>MGSSHHHHHHGSGENLYFQSNQPLKIVVPFSAGGTADVLPRLVAEKIRADYAGGVIIENKPGAGGNIGADLVFRAPPDGMTVLASPPGPIAINHNLYQKLSFDPTRWVPVTILATVPNVLVINPKLPVKSLGEFIAYAKANPKKVTVATQGDGSTSHLTAAMFMQLTGTELTVIPYKGTA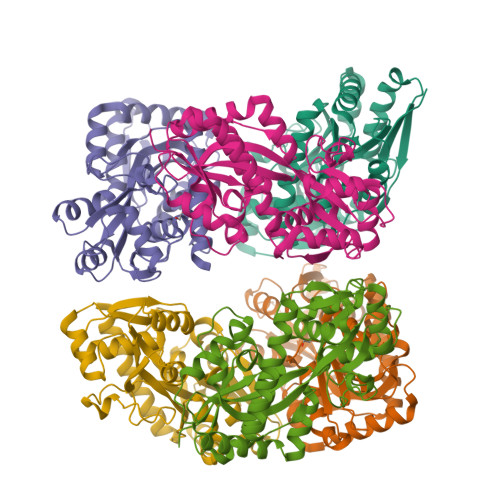PALIDLIGGNVDVFFDNISSSATYHQAGKVRILAVADEQRSQILPQVPTFAEQQWPAMQAVTFFSVVAPPGTSAEIAQKLQKQMALALSSNDIRKHFQEQGAVPCGWDPSKTAQFIRQETEKWKKVLKAANVKL[6x]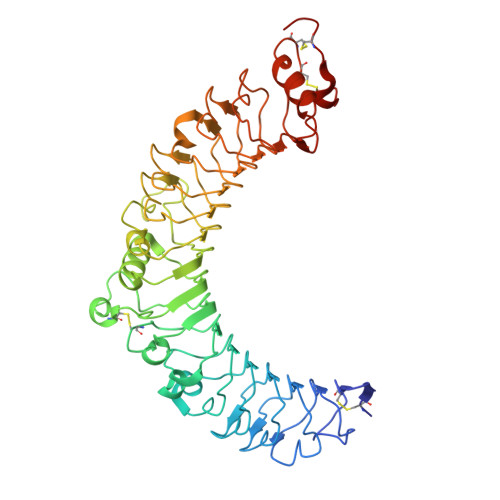> ADPGTSECSVIGYNAICINRGLHQVPELPAHVNYVDLSLNSIAELNETSFSRLQDLQFLKVEQQTPGLVIRNNTFRGLSSLIILKLDYNQFLQLETGAFNGLANLEVLTLTQCNLDGAVLSGNFFKPLTSLEMLVLRDNNIKKIQPASFFLNMRRFHVLDLTFNKVKSICEEDLLNFQGKHFTLLRLSSITLQDMNEYWLGWEKCGNPFKNTSITTLDLSGNGFKESMAKRFFDAIAGTKIQSLILSNSYNMGSSFGHTNFKDPDNFTFKGLEASGVKTCDLSKSKIFALLKSVFSHFTDLEQLTLAQNEINKIDDNAFWGLTHLLKLNLSQNFLGSIDSRMFENLDKLEVLDLSYNHIRALGDQSFLGLPNLKELALDTNQLKSVPDGIFDRLTSLQKIWLHTNPWDCSCPRIDYLSRWLNKNSQKEQGSAKCSGSGKPVRSIICPTSASLVPR> ESQPDPKPDELHKSSKFTGLMENMKVLYDDNHVSAINVKSIDQFLYFDLIYSIKDTKLGNYDNVRVEFKNKDLADKYKDKYVDVFGANYYYQCYFSKKTNDINSHQTDKRKTCMYGGVTEHNGNQLDKYRSITVRVFEDGKNLLSFDVQTNKKKVTAQELDYLTRHYLVKNKKLYEFNNSPYETGYIKFIENENSFWYDMMPAPGDKFDQSKYLMMYNDNKMVDSKDV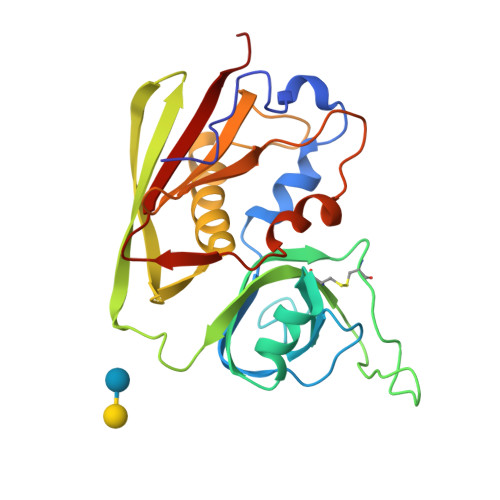KIEVYLTTKKK The icosahedral capsid contains 60 copies of a protomeric unit composed of four proteins, VP1-4. Enteroviruses are unique in harbouring a lipid molecule (pocket factor) within a pocket in the VP1 β-barrel, which lies below the surface of a deep depression encircling each fivefold axis, termed the canyon. The binding of such receptors can trigger pocket factor release and viral expansion, leading to externalization of the N-terminus of VP1 followed by VP4 to form a pore in the endo/lysosome membrane through which the genome is thought to be subsequently released. Here, we have determined three cryo-EM structures following mixing of CV-A10 Kowalik strain with KRM1: the CV-A10 mature virus, a disassembly intermediate A-particle and the mature virus in complex with KRM1.

Of the three bands visible on the gradient, the material used in the cryo-EM analysis was derived exclusively from the lower band. Thermofluor and cryo-EM analysis showed that these particles were mature virus rather than A-particles (“Methods” section and Supplementary Fig. 2). As expected, the structure of CV-A10 Kowalik maintains the typical enterovirus architecture and surface topography but a signature of CV-A10 viruses is an extended VP1 BC loop that, together with the absence of helical structure in the VP1 GH loop, widens the front part of the canyon whilst the extended VP2 EF loop is bent inwards narrowing the rear of the canyon and the VP3 C-terminus protrudes into the base of the canyon. This contributes to a distinct electrostatic surface potential compared to HFMD viruses from other receptor sub-groups. A distinguishing feature of this strain is ordered density allowing the whole of a 13-residue long helix at the N-terminal end of VP1 to be built. This structure lies underneath the VP2 helices that abut at the twofold axes, in a similar position to, but eight residues longer than, the corresponding helix found in EV-A71 and CV-A16. Internally, the N-terminal portion of VP4 is disordered in CV-A10 Kowalik, but residues 18–28 are observed to cross to an adjacent biological protomer in strain SJZ10-1740T/HeB/CHN/201014. Disordered RNA density is visible within the particle, the outer portion rather closely packed against the inside of the capsid.

> GDPVEDIIHDALSSTVRRAITSGQDVNTAAGTAPSSHRLETGRVPALQAAETGATSNATDENMIETRCVMNRNGVLEATISHFFSRSGLVGVVNLTDGGTDTTGYAVWDIDIMGFVQLRRKCEMFTYMRFNAEFTFVTTTENGEARPFMLQYMYVPPGAPKPTGRDAFQWQTATNPSVFVKLTDPPAQVSVPFMSPASAYQWFYDGYPTFGQHPETSNTTYGQCPNNMMGTFAVRVVSRVASQLKLQTRVYMKLKHVRAWIPRPIRSQPYLLKNFPNYDSSKITYSARDRASIKQANM;> SPSVEACGYSDRVAQLTVGNSSITTQEAANIVLAYGEWPEYCPDTDATAVDKPTRPDVSVNRFYTLDSKMWQENSTGWYWKFPDVLNKTGVFGQNAQFHYLYRSGFCLHVQCNASKFHQGALLVAVIPEFVLAGRGSNTKPNEAPHPGFNTTFPGTAGASFNDPYVLDSGVPLSQSLIYPHQWINLRTNNCATIIVPYINAVPFDSAINHSNFGLIVVPVSPLKYSSGATTAIPITVTIAPLNSEFGGLRQAVSQ;> GLPTELRPGTNQFLTTEDDTAAPILPGFSPTPSIHIPGEVRSLLELCRVETILEVNNTTDATGLNRLLIPVSAQNKADELCAAFMVDPGRIGPWQSTLVGQICRYYTQWSGSLKVTFMFTGSFMATGKMLIAYSPPGSAQPANRETAMLGTHVIWDFGLQSSVSLVIPWISNTHFRTAKTGGNYDYYTAGVVTLWYQTNYVVPPETPGEAYIIAMGAAQDNFTLKICKDTDEVTQQAVLQ;> MGAQVSSQRSGSHETGNVATGGSTINFTNINYYKDSYAASASRQDFTQDPKKFTQPVLDSIRELSAPLN> GSHMGDQRFGDLVFRQLAPNVWQHTSYLDMPGFGAVASNGLIVRDGGRVLVVDTAWTDDQTAQILNWIKQEINLPVA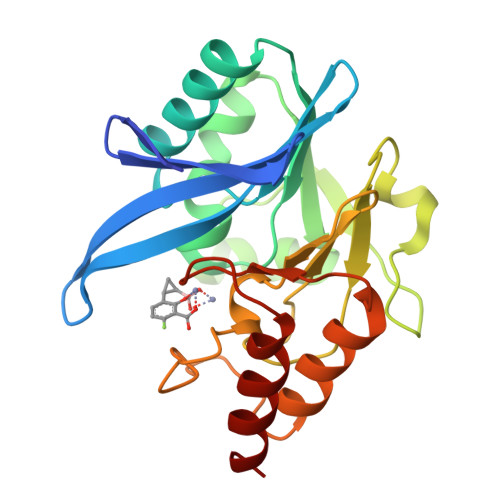LAVVTHAHQDKMGGMDALHAAGIATYANALSNQLAPQEGMVAAQHSLTFAANGWVEPATAPNFGPLKVFYPGPGHTSDNITVGIDGTDIAFGGCLIKDSKAKSLGNLGDADTEHYAASARAFGAAFPKASMIVMSHSAPDSRAAITHTARMADKLR>MATPASGALLQQMNLASQSLNYELSFISINKQGVESLRYRHARLDNRPLAQLLQMDGPRREVVQRGNEISYFEPGLEPFTLNGDYIVDSLPSLIYTDFKRLSPYYDFISVGRTRIADRLCEVIRVVARDGTRYSYIVWMDTESKLPMRVDLLDRDGETLEQFRVIAFNVNQDISSSMQTLA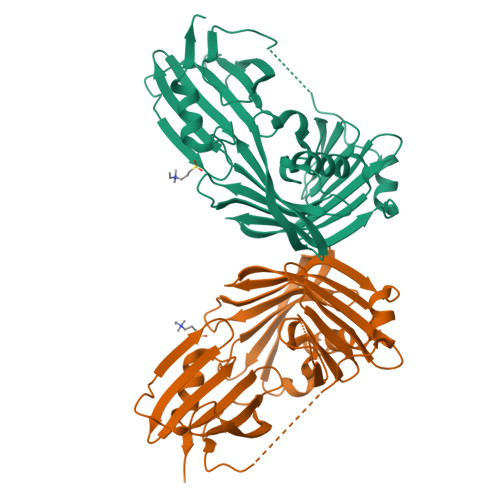KANLPPLLSVPVGEKAKFSWTPTWLPQGFSEVSSSRRPLPTMDNMPIESRLYSDGLFSFSVNVNRATPSSTDQMLRTGRRTVSTSVRDNAEITIVGELPPQTAKRIAENIKFGAAQHHHHHH[2x]>GPATPLSATAALRDGAGQVVGSARFVQQGAGVQVTVDVRGLTPGMHGMHVHEFGRCTPGVDPAVNKVVPFGAAGGHFDPSMSRNHDTPQTDNKHGHGGDTPMLSVGADGVGKASFTSTKISLTGENGILNRSLVIHANPDDYKTDPAGMSGARERCGVIVRDGLSVRDYALPGPVDHPEGVAYDAKKGLIYTGSAQNGTIYAINAQSGAVTKFQEGGAYGRQVALGLKVDPQGRLWIAGGAQGTVSILTPDGMTLAVLETPKSPRPYINDLVLAPDGNFYVTDSSRPVIFRVDKALKLTAWLDLAGTPIKYGPGVNLNGIAATPDGKYLLAVQLNTGELWRIDLKTKAVKKVMDGLVNGDGLLLDGRTLYVARNKDQVVAKVSLSADYGSGQLVAQEPLNGLRFPATLAKVGNDLVVTQAQLDRIGGTPETPFKLTRFAKF[2x]

Here, we show a unique type of Cu/Zn-SOD from Deinococcus radiodurans (DrSOD) with an additional β-propeller domain. In this study, we revealed a unique structure of DrSOD, where the Cu/Zn-SOD domain (DrSODSOD) is fused with a six-bladed β-propeller domain (DrSODβ-pro). Each domain utilizes a different metal ion—a copper and zinc ion for DrSODSOD and a calcium ion for DrSODβ-pro—to independently drive superoxide dismutation and lactone hydrolysis, respectively. pmcCu/Zn-superoxide dismutase (Cu/Zn-SOD) is an antioxidant enzyme found across a wide range of organisms, where it plays a role in detoxifying superoxide radicals by catalyzing their dismutation into molecular oxygen and hydrogen peroxide.

To elucidate the structure of calcium-free DrSOD, we also analyzed the DrSOD crystallized in the presence of equimolar copper and zinc ions but without the addition of calcium ions. Under these conditions, crystallization occurred at a relatively acidic pH (pH 4.0), which likely hindered the zinc binding (top). Also, the zinc-binding loop, electrostatic loop, and S-S subloop in DrSODSOD were not determined, possibly due to significant structural fluctuations (top). Nevertheless, the overall structure of calcium-free DrSOD crystallized under acidic conditions was nearly superimposable with that of the calcium-bound form crystallized at pH 8.0, with an RMSD of 0.305 Å between calcium-free and calcium-bound DrSOD in chain A. Both crystal structures contain two molecules in the asymmetric unit with no significant differences between them; therefore, the comparison was focused on chain A in both structures. The side chain of Asp339 in the calcium-free DrSOD adopted an orientation away from the center of the β-propeller, resembling the orientation away from the calcium ion in the calcium-bound form of DrSOD (bottom). While it remains uncertain whether the crystals obtained in the presence of calcium ions contain a mixture of calcium-bound and calcium-free DrSOD molecules, the orientation of the Asp339 side chain pointing toward the calcium ion was exclusively observed in the calcium-bound form. These observations thus suggest that Asp339 plays a role in the binding of the calcium ion.> GLEDDLVEVIVDKAQQTLASIKSDSKHTQKVPSL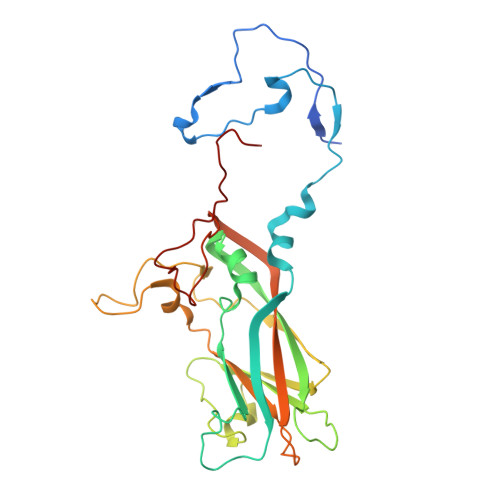TANETGATLPTTPSDSVETRTTLMHYTGSETTLENFLGRAACVHVVEIVNKRPTDTEEHRMQLLFNNWKINLSSLVQLRRKLEMFTYVRFDSEYTIIATSSQPNEAKFSSNLTIQAMFIPPGAPNPKKWDDYTWQSATNPSVFFNVGKSARFSVPYLGIASAYNCFYDGYSHDNSTTPYGINVLNHMGSMAFRVVNEHDNHTTHVKVRVYHRAKHIRAWVPRAPRALEYLHIGRTNYKQSPQNPIKTRKTISTY> MIQGVIQKIAGPAVIAKGMLGARMYDICKVGEEGLVGEIIRLDGDTAFVQVYEDTSGLKVGEPVVSTGLPLAVELGPGMLNGIYDGIQRPLERIREKTGIYITRGVVVHALDREKKWAWTPMVKPGDEVRGGMVLGTVPEFGFTHKILVPPDVRGRVKEVKPAGEYTVEE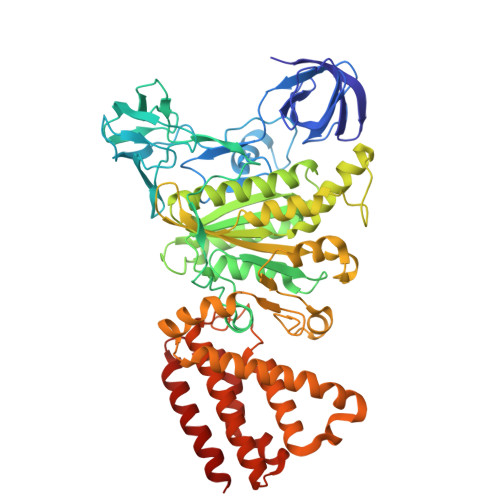PVVVLEDGTELKMYHTWPVRRARPVQRKLDPNTPFLTGMRILDVLFPVAMGGTAAIPGPFGAGKSVTQQSLAKWSNADVVVYVGCGERGNEMTDVLVEFPELTDPKTGGPLMHRTVLIANTSNMPVAAREASIYVGVTIAEYFRDQGFSVALMADSTSRWAEALREISSRLEEMPAEEGYPPYLAARLAAFYERAGKVITLGGEEGAVTIVGAVSPPGGDMSEPVTQSTLRIVGAFWRLDASLAFRRHFPAINWNGSYSLFTSALDPWYRENVAEDYPELRDAISELLQREAGLQEIVQLVGPDALQDAERLVIEVGRIIREDFLQQNAYHEVDAYCSMKKAYGIMKMILAFYKEAEAAIKRGVSIDEILQLPVLERIGRARYVSEEEFPAYFEEAMKEIQGAFKALA>[3x]MHAINIAFFDLIMPVEKTLLILKPDAVARG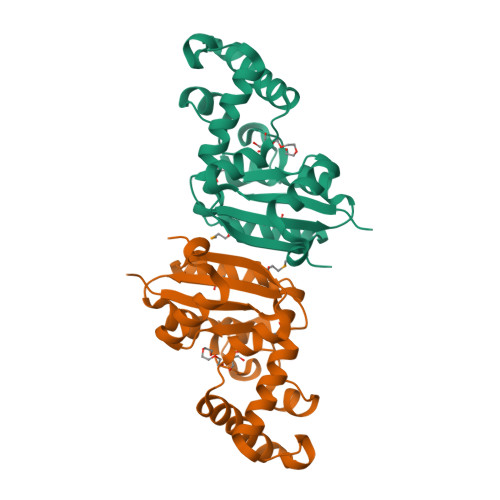LVDEIISRFKKAGLKIVALKMVKASPEEIERFYPSSEEWLQSAGQKLLKAYQELGIDPRAKIGTDDPVEVGRIIKRNLVKYMTSGPNVVMVLKGNRAVEIVRKLVGPTSPHSAPPGTIRGDYSIDSPDLAAEEGRVVFNLVHASDSPSEAEREIRFWFREEEVLE>EAEATDPNGYIVFCPCMGRFGNQVDQFLGVLAFAKALDRTLVLPNFIEFKHPETKMIPFEFLFQVGTVAKYTRVVTMQEFTKKIMPTVWPPEKRKAFCWTPRQAIYDKSAEPGCHSKEGNPFGPYWDQIDVSFVGDEYFGDIPGGFDLNQMGSRKKWLEKFPSEEYPVLAFSSAPAPFPSKGKVWSIQKYLRWSSRITEQAKKFISANLAKPFVAVHLRNDADWVRVCEHIDTTTNRPLFASEQCLGEGHHLGTLTKEICSPSKQQILEQIVEKVGSIGAKSVFVASDKDHMIDEINEALKPYEIEAHRQEPDDMYTSLAIMGRADLFVGNCVSTFSHIVKRERDHAGQSPRPSAF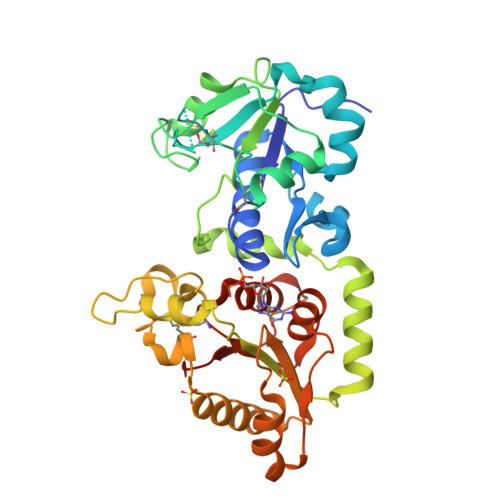FGIRAV[2x]>[2x]MKEFAYSEPCLDKEDKKAVLEVLNSKQLTQGKRSLLFEEALCEFLGVKHALVFNSATSALLTLYRNFSEFSADRNEIITTPISFVATANMLLESGYTPVFAGIKNDGNIDELAL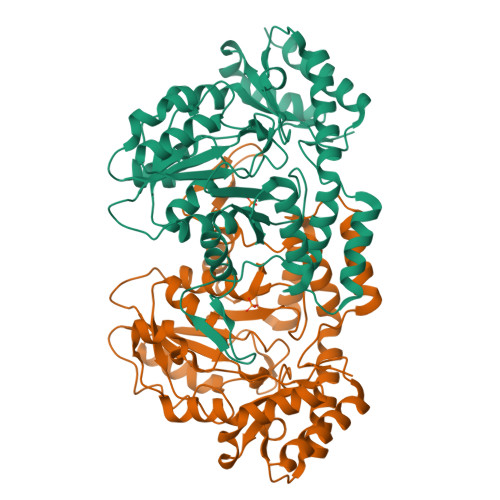EKLINERTKAIVSVDYAGKSVEVESVQKLCKKHSLSFLSDSSHALGSEYQNKKVGGFALASVFSFHAIKPITTAEGGAVVTNDSELHEKMKLFRSHGMLKKDFFEGEVKSIGHNFRLNEIQSALGLSQLKKAPFLMQKREEAALTYDRIFKDNPYFTPLHPLLKDKSSNHLYPILMHQKFFTCKKLILESLHKRGILAQVHYKPIYQYQLYQQLFNTAPLKSAEDFYHAEISLPCHANLNLESVQNIAHSVLKTFESFKIE> MAHHHHHHMTQSSTPVCVITGSASGIGAATALRFAQAGWSVAIGNFDDSTRDAASTVEALCRDAGAQTLIFDADVGKDADCRHAVDMVASRWQRIDALINCAGTTRVIPHNAFDQIDDFEFERVYRVNLIGLYQMTRAAVPLLRESASATRSTSVVNVSSLAGLNGTGSSIAYAASKGAVNTLTLSLARNLAPHIRVNALAPGMVDDGLLLRVLDAAAYDGVLSRMTESAPLKRVSRPAEIAELAWFLTAHAPAITGQVIAAENG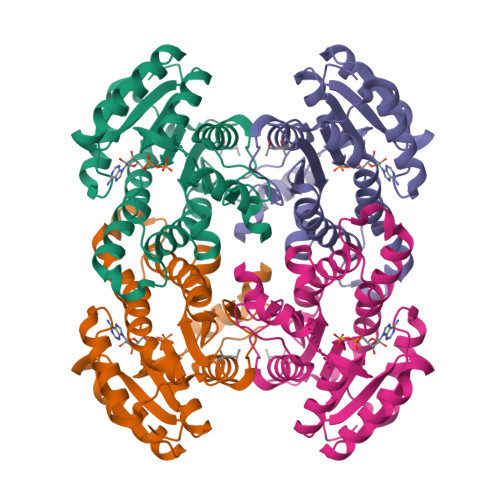LLLGGA> MAGAPHPHTYMGWWGSLGSPKQKYITQYTISPYAAKPLKGAAYNAVFNTFRRTKNQ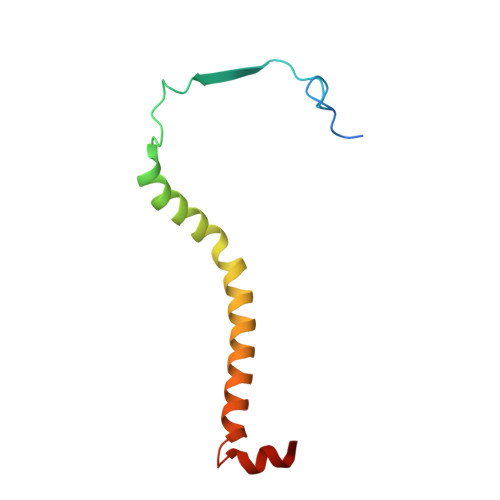FLYVAIPFVVVWSIWTRARDYNEYLYTKEGREELERVNV(2R)-hexane-1,2-diol | C6 H14 O2 | 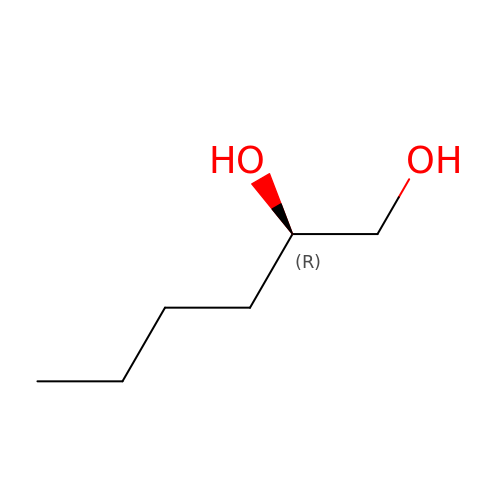FHKSXSQHXQEMOK-ZCFIWIBFSA-N>MGSSHHHHHHSSENLYFQGHMWVKILSVVGARPQFIKAAAVSRVLRASPGVREVLVHTGQHYDDNMSQVFFEELEIPDPDYHLGIGGGTHGQNTGRMLEAIEGVLLKEKPDWVLVYGNTDSTLAGALAAVKLHIPVAHVEAGLRSFNRRMPEEINRILTDHASDLLFAPTETAVQNLLREGIPENRIHLVGDVMYDAALHYGAKAERKSRILERLGLQAKGYVLATIHRAENTDDQERLRVILEALAEVHQEVPVVFPVHPRTRKRAEAFGLGSYLEKVVALEPVGYLDMVMLEKNARLIVTDSGGVQKEAYFYRVPCVTVREETEWVELLKAEWNYLAAPQNAKDLALTILHRMRTKGVEIDLYGDGRASQKISDFLRKVGIRT[2x]

The final step in the pathway is catalyzed by a 2-epimerase, which utilizes UDP-2,3-diacetamido-2,3-dideoxy-d-glucuronic acid as its substrate. The focus of this investigation is on the ORF WP_011172736, which we demonstrate encodes for a 2-epimerase. We have also demonstrated that the T. thermophilus enzyme is allosterically regulated by UDP-GlcNAc. Whereas the sugar 2-epimerases that function on UDP-GlcNAc have been the focus of past biochemical and structural analyses, this is the first detailed investigation of a 2-epimerase that specifically utilizes UDP-2,3-diacetamido-2,3-dideoxy-d-glucuronic acid as its substrate.

Given the unexpected presence of UDP-GlcNAc in structure 4, we next conducted crystallization trials that included both UDP-GlcNAc3NAcA and UDP-GlcNAc. Crystals were obtained at pH 9.0 (structure 6) and pH 6.0 (structure 7). Both models at pH 9.0 and 6.0 were determined to 2.2 Å resolution and refined to overall R-factors of 19.4% and 17.5%, respectively. Regardless of pH, each subunit of the dimer contained both UDP-GlcNAc3NAcA in the active site and UDP-GlcNAc in the auxiliary binding pocket.> MGVNAVHWFRKGLRLHDNPALKECIQGADTIRCVYILDPWFAGSSNVGINRWRFLLQCLEDLDANLRKLNSRLFVIRGQPADVFPRLFKEWNITKLSIEYDSEPFGKERDAAIKKLATEAGVEVIVRISHTLYDLDKIIELNGGQPPLTYKRFQTLVSKMEPLEMPADTITSDVIGKCMTPLSDDHDEKYGVPSLEELGFDTDGLSSAVWPGGETEALTRLERHLERKAWVANFERPRMNANSLLASPTGLSPYLRFGCLSCRLFYFKLTDLYKKVKKNSSPPLSLYGQLLWREFFYTAATNNPRFDKMEGNPICVQIPWDKNPEALAKWAEGRTGFPWIDAIMTQLRQEGWIHHLARHAVACFLTRGDLWISWEEGMKVFEELLLDADWSINAGSWMWLSCSSFFQQFFHCYCPVGFGRRTDPNGDYIRRYLPVLRGFPAKYIYDPWNAPEGIQKVAKCLIGVNYPKPMVNHAEASRLNIERMKQIYQQLSRYRGLGLLASVPSNSNGNGGLMGYAPGENVPSCSSSGNGGLMGYAPGENVPSCSGGNC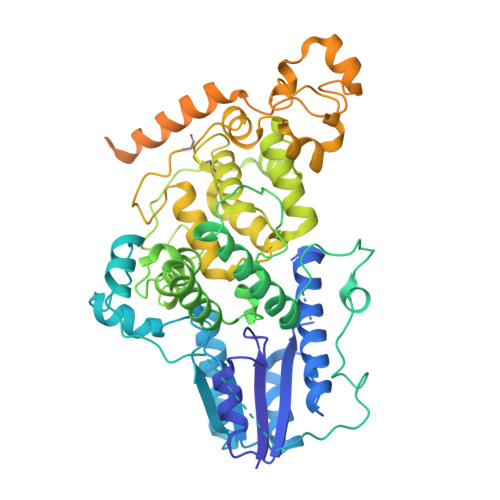SQGSGILHYAHGDSQQTHSLKQGRSSAGTGLSSGKRPSQEEDAQSVGPKVQRQSSNAAALEHHHHHH>[3x]GPHMKHPLMNVWTLWYLENDRSKSWEDMQNEITSFDTVEDFWSLYNHIKPPSEIKLGSDYSLFKKNIRPMWEDAANKQGGRWVITLNKSSKTDLDNLWLDVLLCLIGE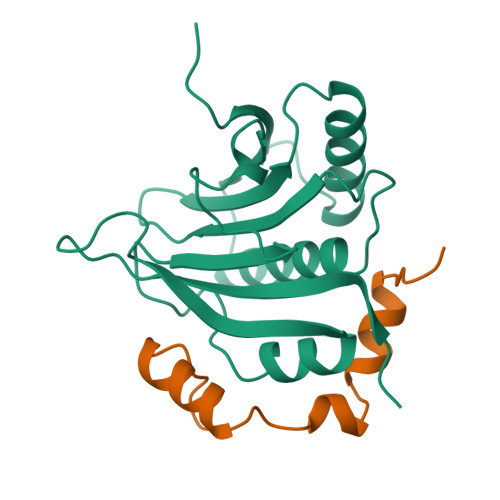AFDHSDQICGAVINIRGKSNKISIWTADGNNEEAALEIGHKLRDALRLGRNNSLQYQLHKDTMVKQGSNVKSIYTL;>[3x]GPHMLERYSKVDLLALRYSPLSQTPPGIELEGRLRRMNIWRTGS> HPLL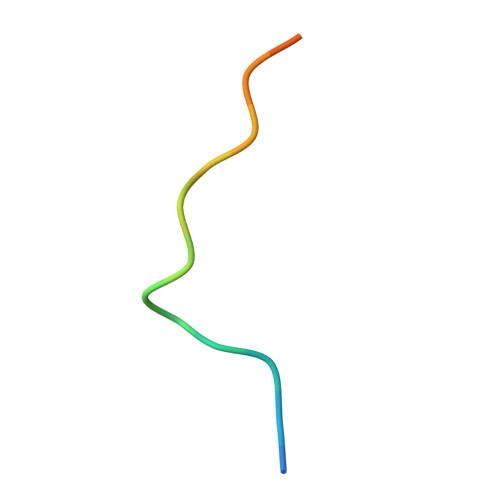NPSALEFNPSQTY Here, we report a cryogenic electron microscopy (cryo-EM) structure of the full-length human HECT HACE1, along with solution-based conformational analyses by small-angle X-ray scattering and hydrogen–deuterium exchange mass spectrometry. Structure-based functional analyses in vitro and in cells reveal that the activity of HACE1 is stringently regulated by dimerization-induced autoinhibition. By contrast, HECTs form a thioester-linked intermediate with Ub before transferring it to a substrate. A RHO-family GTPase, RAC1 cycles between inactive, GDP-bound and active, GTP-bound forms, allowing for spatiotemporal regulation of its interactions and functions.

We determined a cryo-EM structure of the HACE1 dimer at 4.7 Å resolution, using AlphaFold2 (AF2)-based predictions as a starting point for model building. Each subunit of the dimer consists of a C-terminal HECT domain, flanked by an α-helical ‘middle domain’ (MID), seven ankyrin repeats (ANKs) and an N-terminal α-helix (‘N-helix’; residues 1–21). The MID and ANKs form a concave platform, above which the HECT domain leans peripherally. The subunits are arranged in a closed, head-to-tail fashion, giving rise to a ring made up of two sets of ANKs, MIDs and small wings of the HECT N-lobes (for HECT domain architecture). The large wings of the N-lobes are juxtaposed on the inside of the ring, giving rise to a yin–yang-like overall arrangement. The catalytic C-lobes protrude above the platforms, with one adopting an inverted-T conformation (molecule A). In the cryo-EM structure, dimerization is largely mediated by contacts of the N-helix of one subunit with the small wing of the HECT N-lobe of the other, with minor contributions from the N-terminal ANK. The structure of HACE1 FL provides a rationale for how dimerization inhibits the two-step catalytic cycle: at the subunit interface, the N-helix engages intermolecularly with a region of the HECT N-lobe that coincides with the conserved E2 binding site. Although this site, including a key phenylalanine (Phe715), is conserved in HACE1, it is occluded in the dimer. The binding mode is incompatible with the HACE1 dimer, highlighting another layer of autoinhibition.

>[2x]GMERAMEQLNRLTRSLRRARTVELPEDNETAVYTLMPMVMADQHRSVSELLSNSKFDVNYAFGRVKRSLLHIAANCGSVECLVLLLKKGANPNYQDISGCTPLHLAARNGQKKCMSKLLEYSADVNICNNEGLTAIHWLAVNGRTELLHDLVQHVSDVDVEDAMGQTALHVACQNGHKTTVQCLLDSGADINRPNVSGATPLYFACSHGQRDTAQILLLRGAKYLPDKNGVTPLDLCVQGGYGETCEVLIQYHPRLFQTIIQMTQNEDLRENMLRQVLEHLSQQSESQYLKILTSLAEVATTNGHKLLSLSSNYDAQMKSLLRIVRMFCHVFRIGPSSPSNGIDMGYNGNKTPRSQVFKPLELLWHSLDEWLVLIATELMKNKRDSTEITSILLKQKGQDQDAASIPPFEPPGPGSYENLSTGTRESKPDALAGRQEASADCQDVISMTANRLSAVIQAFYMCCSCQMPPGMTSPRFIEFVCKHDEVLKCFVNRNPKIIFDHFHFLLECPELMSRFMHIIKAQPFKDRCEWFYEHLHSGQPDSDMVHRPVNENDILLVHRDSIFRSSCEVVSKANCAKLKQGIAVRFHGEEGMGQGVVREWFDILSNEIVNPDYALFTQSADGTTFQPNSNSYVNPDHLNYFRFAGQILGLALNHRQLVNIYFTRSFYKHILGIPVNYQDVASIDPEYAKNLQWILDNDISDLGLELTFSVETDVFGAMEEVPLKPGGGSILVTQNNKAEYVQLVTELRMTRAIQPQINAFLQGFHMFIPPSLIQLFDEYELELLLSGMPEIDVSDWIKNTEYTSGYEREDPVIQWFWEVVEDITQEERVLLLQFVTGSSRVPHGGFANIMGGSGLQNFTIAAVPYTPNLLPTSSTCINMLKLPEYPSKEILKDRLLVALHCGSYGYTMA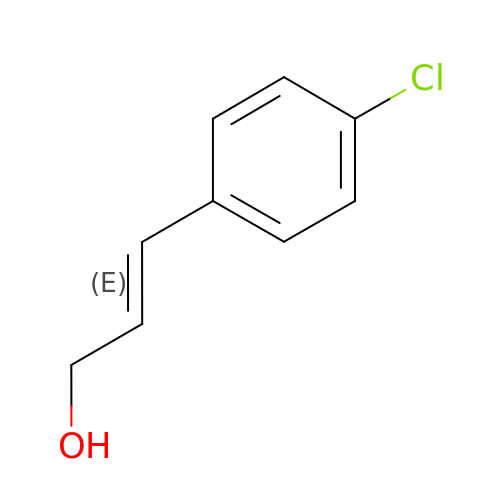(2E)-3-(4-chlorophenyl)prop-2-enal | C9 H9 Cl O | HFMHVOCTLZMPRY-OWOJBTEDSA-N2-[CARBOXY-(2-THIOPHEN-2-YL-ACETYLAMINO)-METHYL]-5-METHYL-3,6-DIHYDRO-2H-[1,3]THIAZINE-4-CARBOXYLIC ACID | C14 H16 N2 O5 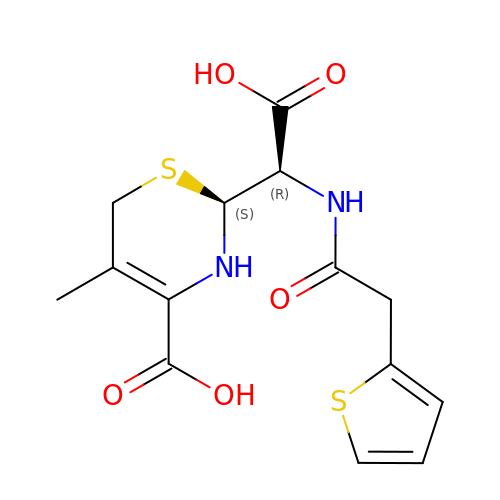S2 | JRYZEMHNDUZNMI-RYUDHWBXSA-N>[3x]GSPGENLKHIITLGQVIHKRCEEMKYCKKQCRRLGHRVLGLIKPLEMLQDQGKRSVPSE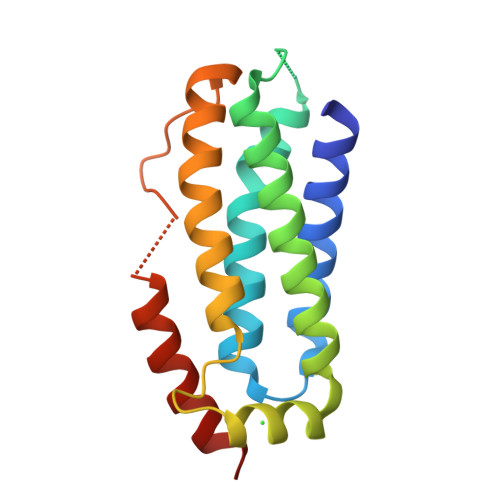KLTTAMNRFKAALEEANGEIEKFSNRSNICRFLTASQDKILFKDVNRKLSDVWKELSLLLQVEQRMPVSPISQGASWAQEDQQDADEDRRAFQM>MIDFGTIATAMVTPFDINGNIDFAKTTKLVNYLIDNGTTAIVVGGTTGESPTLTSEEKVALYRHVVSVVDKRVPVIAGTGSNNTHASIDLTKKATEVGVDAVMLVAPYYNKPSQEGMYQHFKAIAESTPLPVMLYNVPGRSIVQISVDTVVRLSEIENIVAIKDAGGDVLTMTEIIEKTADDFAVY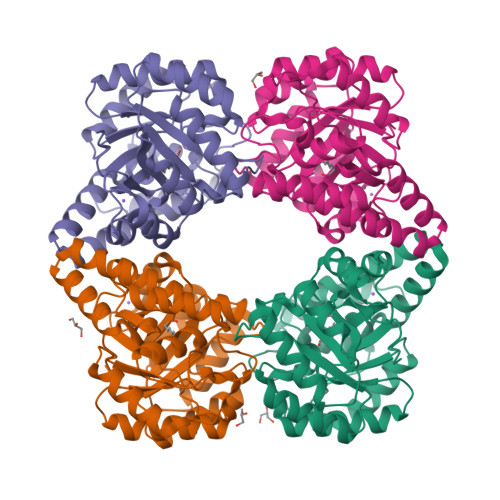SGDDGLTLPAMAVGAKGIVSVASHVIGNEMQEMIAAFQAGEFKKAQKLHQLLVRVTDSLFMAPSPTPVKTALQMVGLDVGSVRLPLLPLTEEERVTLQSVMQSIPR[4x]>CGCGAATXCGCG[2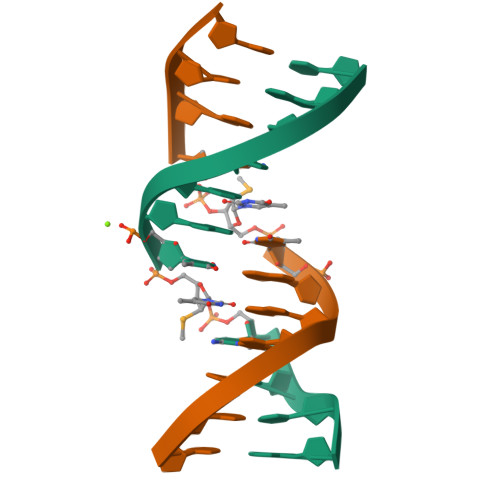x]> GSASNPQTEEVSIKEIAITHHVKEGHEKADPSQFELLKVLGQGSFGKVFLVKKISGSDARQLYAMKVLKKATLKVRDRVRTKMERDILVEVNHPFIVKLHYAFQTEGKLYLILDFLRGGDLFTRLSKEVMFTEEDVKFYLAELALALDHLHSLGIIYRDLKPENILLDEEGHIKLTDFGLSKESIDHEKKAYSFCGTVEYMAPEVVNRRGHTQSADWWSFGVLMFEMLTGTLPFQGKDRKETMTM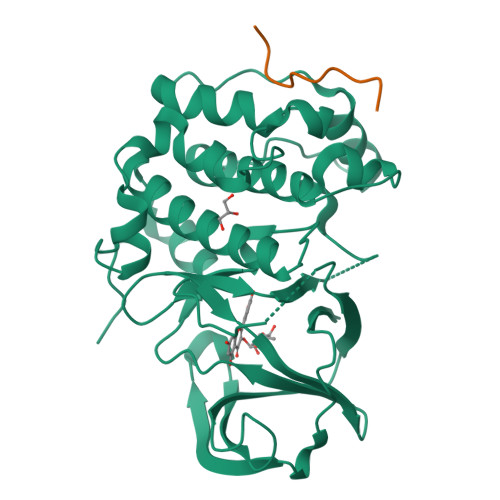ILKAKLGMPQFLSPEAQSLLRMLFKRNPANRLGAGPDGVEEIKRHSFFSTIDWNKLYRREIHPPFKPATGRP;> MEPSQCVEELEDDVFQPED>SLTGEESDTLRKIVLEECLPNQQQNQNPSPCAEVKPNAGYVVLKDLNGPLQYLLMPTYRINGTESPLLTDPSTPNFFWLAWQARDFMSKKYGQPVPDRAVSLAINSRTGRTQNHFHIHISCIRPDVREQLDNNLANISSRWLPLPGGLRGHEYLARRVTESELVQRSPFMM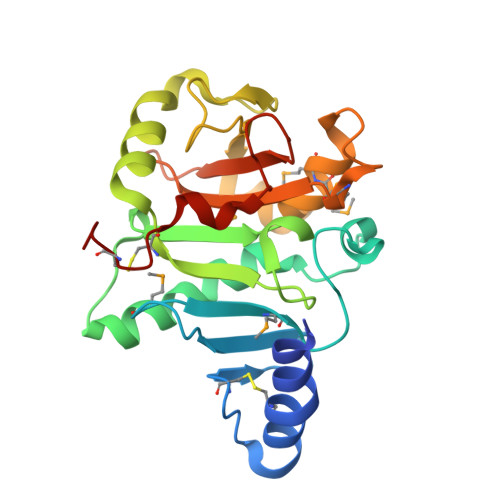LAEEVPEAREHMGSYGLAMVRQSDNSFVLLATQRNLLTLNRASAEEIQDHQCEILR[2x]>MAPQQVNAFSANGSIPSPKEFEGKGKLKLSGRILNVMTSLPLQIISDYDNKTGQYYWDVETVRGNSALYSSQHFLAENKEWETHLIAWTGELINKKKDTSSLTADTLQDDPLYLDEEDKSKIEKKLCDASGTPNIHPVWLLRRDQGRWRKYAENVLWPVFHYIQGQPSDGKAETDAWHDYVKFNEAYLNKIKSVYKPGDIIWIHDYYLLLLPQLLRMEFPNAYIGFFLHVPFPSSEYFRCLSKRSQLLDGMLGADKIGFQSDSFQRHFISCCARVLGCEVNRDSVSAYGTTISVETLPIGIDTEKIEHDAFSSELGVEEKVQALKQVYKGKKLIVGRDRLDKVRGVIQKLEGFEIFLDMYPEWRETVVLIQVSSPGYSHSANVETRVTEIISRINS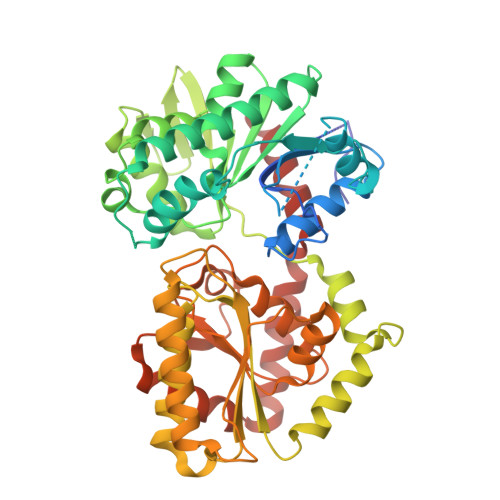KYGNLNHTPVLHYQMRVAKEEYLALLRVADLALITSVRDGMNTTSLEFVICQKYNNSPLILSEFTGTATVLKDAIMVNPWDSVGVAKTINDALMLSTKEKVSLESKLYEKVLSNTVQNWTSTFICDILSHSIVTHSNS[2x]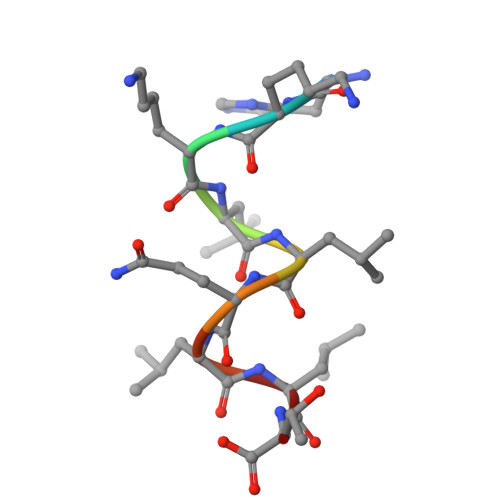> HKKLLQLLT> PKYTKSVLKKGDKTNFPKKGDVVHCWYTGTLQDGTVFDTNIQTSAKKKKNAKPLSFKVGVGKVIRGWDEALLTMSKGEKARLEIEPEWAYGK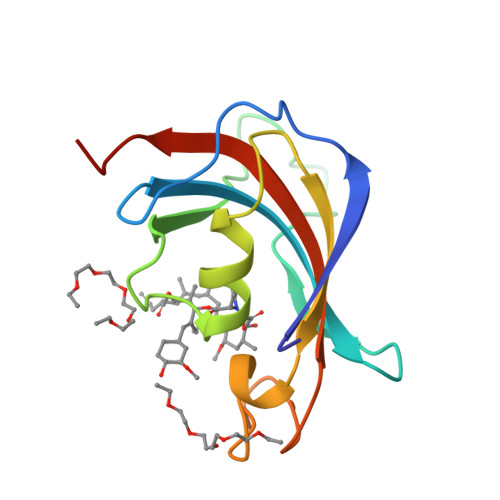KGQPDAKIPPNAKLTFEVELVDIDLEHHHHHH>[2x]TPASRYITDMTIEELSRDWFMLMPKQKVEGPLC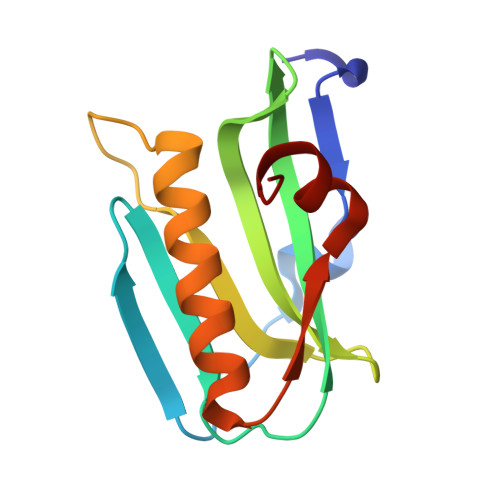IRIDQAIMDKNIMLKANFSVIFDRLETLILLRAFTEEGAIVGEISPLPSFPGHTIEDVKNAIGVLIGGLEWNDNTVRVSKTLQRFAWGS> MDKQI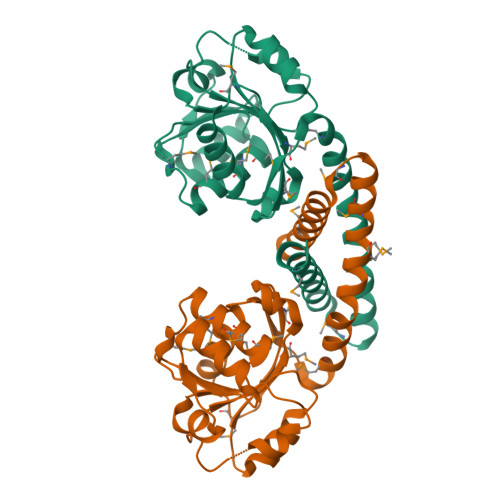GFIGCGNMGMAMIGGMINKNIVSSNQIICSDLNTANLKNASEKYGLTTTTDNNEVAKNADILILSIKPDLYASIINEIKEIIKNDAIIVTIAAGKSIESTENAFNKKVKVVRVMPNTPALVGEGMSALCPNEMVTEKDLEDVLNIFNSFGQTEIVSEKLMDVVTSVSGSSPAYVYMIIEAMADAAVLDGMPRNQAYKFAAQAVLGSAKMVLETGIHPGELKDMVCSPGGTTIEAVATLEEKG Polymeric (p) immunoglobulins (Igs) serve broad functions during vertebrate immune responses. Typically, pIgs are comprised of two to six Ig monomers, each of which contains two heavy chains and two light chains that form one fragment crystallization (Fc) and two antigen-binding fragments (Fabs). To assemble pIgs, plasma cells typically link multiple copies of heavy chains together with a protein called the joining chain (JC); however, incorporation of the JC is variable among species and heavy chain class. Here, we report the cryo-electron microscopy structure of IgM from a teleost (t) species, which does not encode JC.

Guided by previous structural studies indicating that the human IgM constant domain CH2 and Fabs are flexible and poorly resolved in cryo-EM maps, we expressed and purified a truncated teleost IgM heavy chain consisting of CHµ3, CHµ4, and the Tp. We utilized this tIgM Fc (tFcµ) to determine a cryo-EM structure to an average resolution of 2.78 Å. The refined tFcµ structure contains four tFcµ monomers (Fcµ1 to Fcµ4) that lay approximately flat on one plane and include interfaces between Fcµ1 and Fcµ2, Fcµ2 and Fcµ3, Fcµ3 and Fcµ4. Fcµ1 and Fcµ4 are separated by Tp residues, which form a β-sandwich (hereafter termed Tp assembly) comprising two β-strands from each of the four Fcµs. Despite similarity between the two halves of the tetramer, the complex is not symmetrical with respect to all four Fcs; rather, adjacent tFcs are related by distinct angles measuring 81°, 72°, 86°, for Fcµ1 and Fcµ2, Fcµ2 and Fcµ3, Fcµ3 and Fcµ4, respectively. Specifically, the C-terminal 38 residues (residues 411–448; FG loop, G strand and Tp) adopt one of two folds, with chains A and H adopting an A-type fold and chains B-G adopting a B-type fold. In the A-type fold, the FG loop and the G strand include residues 411–416 and 417–426, respectively, and the Tp folds back to form β-sheet interactions with the G strand. In the B-type fold, the FG loop and the G strand instead include residues 411–420 and 421–426, respectively, resulting in Tp β-strand (residues 434–441) being directed away from CHµ4 where they form β-sheet interactions with other Tp(s) rather than the G strand. Interactions between adjacent Fcµ monomers (e.g., Fcµ1-Fcµ2, Fcµ2-Fcµ3, and Fcµ3-Fcµ4) are dominated by a common set of residues in the CHµ4 CD loops, FG loops, and G-strands, forming an interface of ~1360Å2. Cysteine to serine mutation at this residue produced a tFcµ monomer in solution and eliminated evidence of inter-chain disulfide bonding, further suggesting a critical role in tIgM polymeric assembly.

>[8x]HHHHHHHGHLVVITIIEPSLEDMLMNKKAQLVCDVNELVPGFLSVKWENDNGKTLTSRKGVTDKIAILDITYEDWSNGTVFYCAVDHMENLGDLVKKAYKRETGGVPQRPSVFLLAPAEQTSDNTVTLTCYVKDFYPKDVLVAWLVDDEPVERTSSSALYQFNTTSQIQSGRTYSVYSQLTFSNDLWKNEEVVYSCVVYHESMIKSTNIIMRTIDRTSNQPNLVNLSLNVPQRCMAQ> MQGSVTEFLKPRLVDIEQVSSTHAKVTLEPLERGFGHTLGNALRRILLSSMPGCAVTEVEIDGVLHEYSTKEGVQEDILEILLNLKGLAVRVQGKDEVILTLNKSGIGPVTAADITHDGDVEIVKPQHVICHLTDENASISMRIKVQRGRG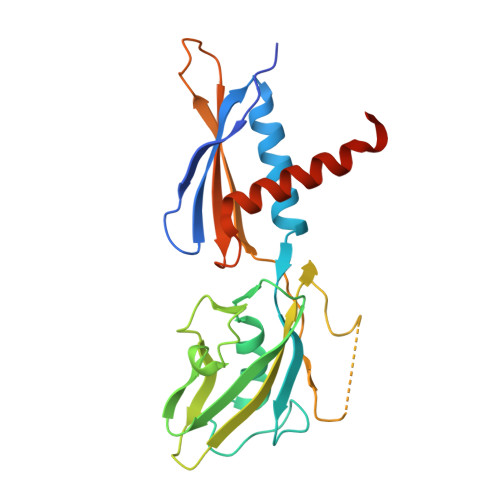YVPASTRIHSEEDERPIGRLLVDACYSPVERIAYNVEAARVEQRTDLDKLVIEMETNGTIDPEEAIRRAATILAEQLEAFVDLEVLFQ>ICNKYKNINVNMKKNNDDTWTDLVKNSSDINKGVLLPPRRKNLF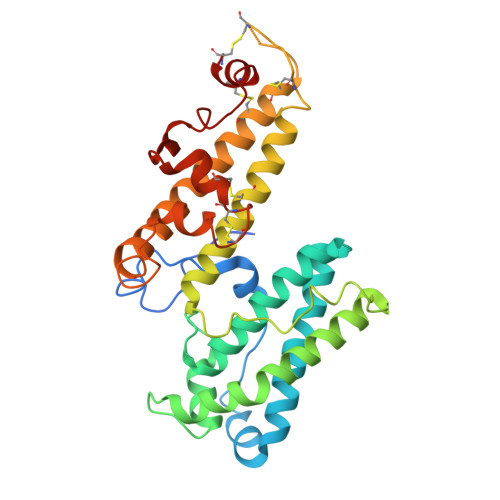LKIDESDICKYKRDPKLFKDFIYSSAISEVERLKKVYGEAKTKVVHAMKYSFADIGSIIKGDDMMENNSSDKIGKILGDGVGQNEKRKKWWDMNKYHIWESMLSGYKHAYGNISENDRKMLDIPNNDDEHQFLRWFQEWTENFCTKRNELYENMVTACNSAKCNTSNGSVDKKECTEACKNYSNFILIKKKEYQSLNSQYDMNYKETKAEKKESPEYFKDKCNGECSCLSEYFKDETRWKNPYETLDDTEVKNNCMCK[2x]>[2x]AEPVYPDQLRLFSLGQGVCGDKYRPVNREEAQSVKSNIVGMMGQWQISGLANGWVIMGPGYNGEIKPGTASNTWCYPTNPVTGEIPTLSALDIPDGDEVDVQWRLVHDSANFIKPTSYLAHYLGYAWVGGNNSQYVGEDMDVTRDGDGWVIRGNNDGGCDGYRCGDKTAIKVSNFAYNLDPDSFKHGDVTQSDRQLVKTVVGWAVNDSDTPQSGYDVTLRYDTATNWSKTNTYGLSEKVTTKNKFKWPLVGETELSIEIAANQSWASQNGGSTTTSLSQSVRPTVPARSKIPVKIELYKADISYPYEFKADVSYDLTLSGFLRWGGNAWYTHPDNRPNWNHTFVIGPYKDKASSIRYQWDKRYIPGEVKWWDWNWTIQQNGLSTMQNNLARVLRPVRAGITGDFSAESQFAGNIEIGAPVPLAADSKVRRARSVDGAGQGLRLEIPLDAQELSGLGFNNVSLSVTPAANQ

Aerolysin is produced by the human pathogen Aeromonas hydrophila as an inactive precursor called proaerolysin. Conversion of proaerolysin to aerolysin involves proteolytic cleavage of a flexible 43-residue loop near the C-terminus. The protein is L-shaped, composed of a continuous globular N-terminal domain, Domain 1, and an elongated region consisting of three discontinuous structural domains. Domain 4 has no known function but contains the CTP, which is folded as 2 anti-parallel β-strands connected by a short α-helix.

Residue His-132 is required for heptamer formation. Our MD-based observations thus suggest that the CTP remains bound to aerolysin upon proteolytic activation of the protoxin. This was confirmed using two independent experimental approaches. First, we determined the structure of the proteolytically processed form of an aerolysin mutant that is unable to form heptamers, namely H132N. Not only was the observed structure very similar to that of wild-type (WT) proaerolysin (root mean square deviation RMSD of 0.74 Å for subunits A and 0.92 Å for subunits B in the dimer), it also contained the CTP, in an essentially identical conformation. The structure of aerolysin H132N and the experiments of binding WT aerolysin-CTP to Nickel beads indeed show that the WT CTP does not come off over a period of several hours, which is inconsistent with a Koff in the order of 10−3 s−1. Thus the binding of the CTP to Domain 4 inhibits oligomerization.> SNAQEPNKDGFYGKFGGRFVPETLMTAVLELEKAYRESQADPSFQEELNQLLRQYVGRETPLYYAKNLTQHIGGAKIYLKREDLNHTGAHKINNALGQVWLAKRMGKKKIIAETGAGQHGVATATAAALFNMECTIYM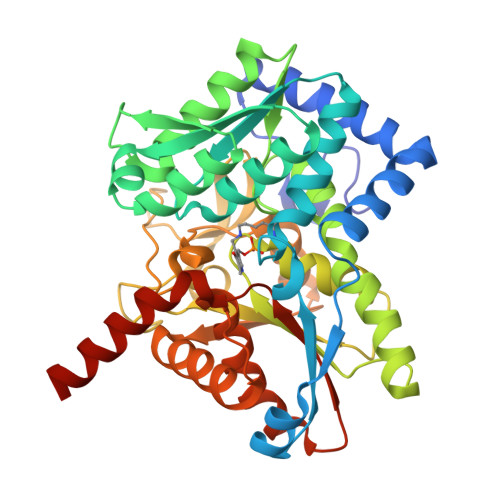GEEDVKRQALNVFRMELLGAKVEAVTDGSRVLKDAVNAALRSWVANIDDTHYILGSALGPHPFPEIVRDFQSVIGREAKQQYRDLTGRDLPDALVACVGGGSNAIGLFHPFVEDESVAMYGTEAAGLGVDTEHHAATLTKGRPGVLHGSLMDVLQDAHGQILEAFSISAGLDYPGIGPEHSHYHDIKRASYVPVTDEEALEGFQLLSRVEGIIPALESSHAIAFAVKLAKELGPEKSMIVCLSGRGDKDVVQVKDRLEADAAKKGEAHA1-(1-methyl-1H-pyrazol-5-yl)methanamine | C5 H9 N3 | 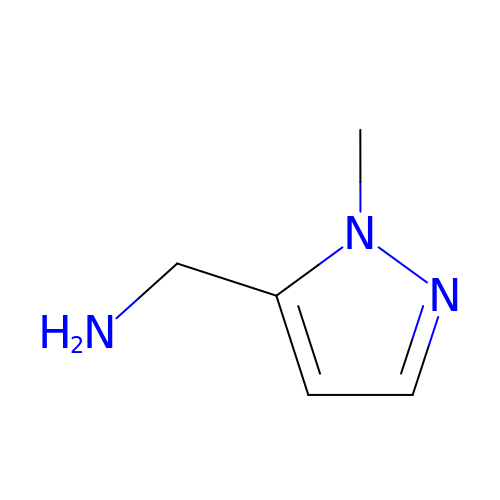XNTFQMKXUFFUQO-UHFFFAOYSA-N> MGSSHHHHHHSSGRENLYFQGHMVKEPGGKHVLCVGAAVLDTLFRVADMPKGEGKVLPYEVLQIAEGMASSAAYAVHRMGGRASLWGAVGDDETGTRILRDLSESGIDTSGMTVAPGARSALSTIIIDNRGERLIVPFYDHRLHEKKRACTPEDIALFDAVLVDVRWPELALDVLTVARALGK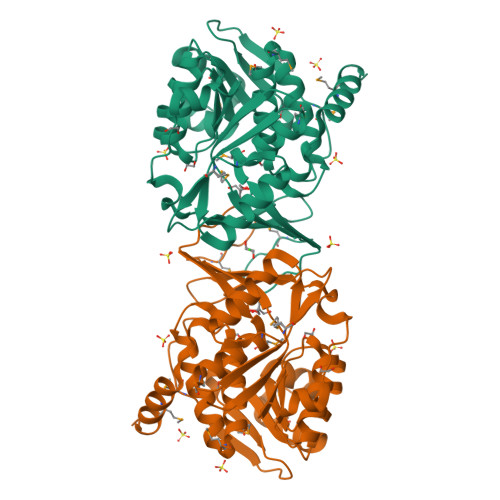PAILDGDVAPVETLEGLAPAATHIVFSEPAATRLTGLETVKDMLPVLHARYPQTFIAVTAGPAGCWWTEADDPTVHFQTTMQVEAVDTLAAGDIFHGTFALAMAEGMQSRAAVRLSSVAAALKCTVFGGRIGAPTREETEEAMRQWLERESEPALRASGS> MSEEKTYKRVEQDDPVPELDIKQGPVRPFIVTDPSAELASLRTMVTLKEKLLVACLAVFTAVIRLHGLAWPDSVVFDEVHFGGFASQYIRGTYFMDVHPPLAKMLYAGVASLGGFQGDFDFENIGDSFPSTTPYVLMRFFSASLGALTVILMYMTLRYSGVRMWVALMSAICFAVENSYVTISRYILLDAPLMFFIAAAVYSFKKYEMYPANSLNAYKSLLATGIALGMASSSKWVGLFTVTWVGLLCIWRLWFMIGDLTKSSKSIFKVAFAKLAFLLGVPFALYLVFFYIHFQSLTLDGDGASFFSPEFRSTLKNNKIPQNVVADVGIGSIISLRHLSTMGGYLHSHSHNYPAGSEQQQSTLYPHMDANNDWLLELYNAPGESLTTFQNLTDGTKVRLFHTVTRCRLHSHDHKPPVSESSDWQKEVSCYGYSGFDGDANDDWVVEIDKKNSAPGVAQE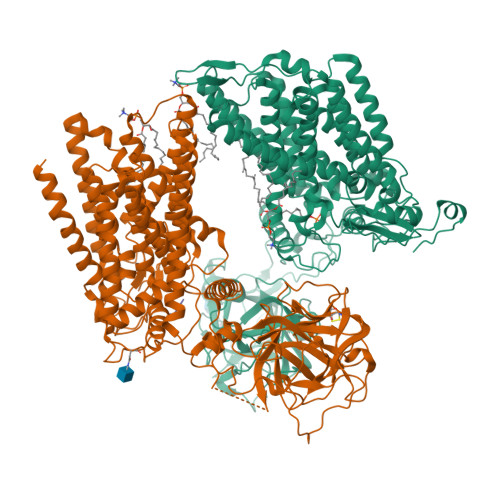RVIALDTKFRLRHAMTGCYLFSHEVKLPAWGFEQQEVTCASSGRHDLTLWYVENNSNPLLPEDTKRISYKPASFISKFIESHKKMWHINKNLVEPHVYESQPTSWPFLLRGISYWGENNRNVYLLGNAIVWWAVTAFIGIFGLIVITELFSWQLGKPILKDSKVVNFHVQVIHYLLGFAVHYAPSFLMQRQMFLHHYLPAYYFGILALGHALDIIVSYVFRSKRQMGYAVVITFLAASVYFFKSFSPIIYGTPWTQELCQKSQWLSGWDYNCNTYFSSLEEYKNQTLTKRESQPAATSTVEEITIEGDGPSYEDLMNEDGKKIFKDTEGNELDPEVVKKMLEEEGANILKVEKRAVLE;> MSSSSSTGYSKNNAAHIKQENTLRQRESSSISVSEELSSADERDAEDFSKEKPAAQSSLLRLESVVMPVIFTALALFTRMYKIGINNHVVWDEAHFGKFGSYYLRHEFYHDVHPPLGKMLVGLSGYLAGYNGSWDFPSGEIYPDYLDYVKMRLFNASFSALCVPLAYFTAKAIGFSLPTVWLMTVLVLFENSYSTLGRFILLDSMLLFFTVASFFSFVMFHNQRSKPFSRKWWKWLLITGISLGCTISVKMVGLFIITMVGIYTVIDLWTFLADKSMSWKTYINHWLARIFGLIIVPFCIFLLCFKIHFDLLSHSGTGDANMPSLFQARLVGSDVGQGPRDIALGSSVVSIKNQALGGSLLHSHIQTYPDGSNQQQVTCYGYKDANNEWFFNRERGLPSWSENETDIEYLKPGTSYRLVHKSTGRNLHTHPVAAPVSKTQWEVSGYGDNVVGDNKDNWVIEIMDQRGDEDPEKLHTLTTSFRIKNLEMGCYLAQTGNSLPEWGFRQQEVVCMKNPFKRDKRTWWNIETHENERLPPRPEDFQYPKTNFLKDFIHLNLAMMATNNALVPDPDKFDYLASSAWQWPTLNVGLRLCGWGDDNPKYFLLGTPASTWASSVAVLAFMATVVILLIRWQRQYVDLRNPSNWNVFLMGGFYPLLAWGLHYMPFVIMSRVTYVHHYLPALYFALIILAYCFDAGLQKWSRSKCGRIMRFVLYAGFMALVIGCFWYFSPISFGMEGPSSNFRYLNWFSTWDIADKQEA;> PYTV> YEKVRIYRMDGSYRSVELKHGNNTTVQQIMEGMRLSQETQQYFTIWICSENLSLQLKPYHKPLQHVRDWPEILAELTNLDPQRETPQLFLRRDVRLPLEVEKQIEDPLAILILFDEARYNLLKGFYTAPDAKLITLASLLLQIVYGNYESKKHKQGFLNEENLKSIVPVTKLKSKAPHWTNRILHEYKNLSTSEGVSKEMHHLQRMFLQNCWEIPTYGAAFFTGQIFTKASPSNHKVIPVYVGVNIKGLHLLNMETKALLISLKYGCFMWQLGDTDTCFQIHSMENKMSFIVHTKQAGLVVKLLMKLNGQLMPTERNS;> MREYKLVVLGSGGVGKSALTVQFVQGIFVEKYDPTIEDSYRKQVEVDAQQCMLEILDTAGTQQFTAMRDLYMKNGQGFALVYSITAQSTFNDLQDLREQILRVKDTDDVPMILVGNKCDLEDERVVGKEQGQNLARQWNNCAFLESSAKSKINVNEIFYDLVRQINR

Herein, we characterize the 2-hydroxy-1-naphthaldehyde (HNA) fragment as a targeted covalent reversible ligand of a noncatalytic lysine (Lys720) of the Krev interaction trapped 1 (KRIT1) protein. The PPI between HEG1 and KRIT1 is believed to play an important role in controlling vascular development and permeability under normal and pathological conditions. The HEG1 binding domain of KRIT1 features three lysines, namely Lys475, Lys720, and Lys724; based on point mutation studies, these residues are essential for the interaction between HEG1 and KRIT1.14 The HNA was found to form a reversible imine adduct with Lys720, and SAR studies indicated that the HNA is the smallest/simplest 2-hydroxy-arylaldehyde that inhibits the HEG1-KRIT1 PPI. However, the interaction of HNA within the HEG1 binding pocket of KRIT1 induces proximity of the aldehyde moiety with the ε-amino group of Lys720, resulting in the specific targeting of this amino acid residue.

To evaluate the potential of the HNA as a site-directing fragment to identify HEG1-KRIT1 PPI inhibitors with potentially improved binding affinity and inhibition activity, we synthesized and screened a series of HNA derivatives bearing substitutions at the C6 or C7 position of the naphthalene ring. The C6 and C7 positions were selected for substitutions as an analysis of the available HNA-KRIT1 co-crystal structure indicated that these two positions may provide opportunities for analogs with improved complementarity to the HEG1 binding region of KRIT1. The co-crystal structures of 3, 5, and 6 in complex with KRIT1 revealed that these compounds exhibit similar binding modes as the parent HNA fragment, including the presence of the imine adduct between the aldehyde moiety of the HNA derivative and the ε-amino group of Lys720. However, compared to the unsubstituted HNA, derivatives 3, 5, and 6 established additional interactions with KRIT1. Additionally, both furan derivatives 5 and 6 were involved in hydrogen−π interactions with KRIT1 Gln473. Interestingly, the binding positions in the three crystal structures appeared nearly identical with the HNA binding pose generated in the MD simulations. Thus, the X-ray and activity data indicate that the binding affinity of the HNA for KRIT1, and the consequent inhibition activity of this fragment in the HEG1–KRIT1 PPI assay, respond to elements of SARs, and in turn highlight the importance of structure complementarity and templating effects in promoting the formation of specific and relatively stable imine adducts with KRIT1 Lys720.> MNSPVDAPKWPRQIPYIIASE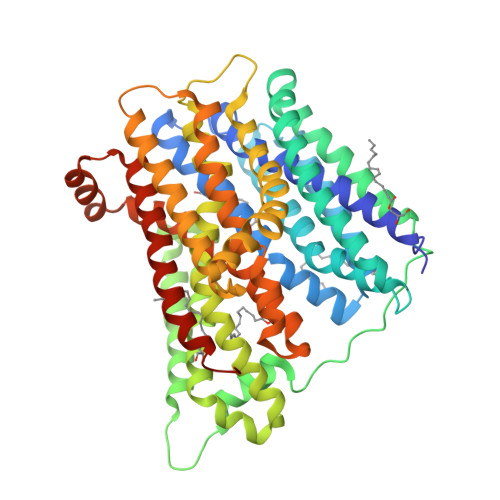ACERFSFYGMRNILTPFLMTALLLSIPEELRGAVAKDVFHSFVIGVYFFPLLGGWIADRFFGKYNTILWLSLIYCVGHAFLAIFEHSVQGFYTGLFLIALGSGGIKPLVSSFMGDQFDQSNKSLAQKAFDMFYFTINFGSFFASLSMPLLLKNFGAAVAFGIPGVLMFVATVFFWLGRKRYIHMPPEPKDPHGFLPVIRSALLTKVEGKGNIGLVLALIGGVSAAYALVNIPTLGIVAGLCCAMVLVMGFVGAGASLQLERARKSHPDAAVDGVRSVLRILVLFALVTPFWSLFDQKASTWILQANDMVKPQWFEPAMMQALNPLLVMLLIPFNNFVLYPAIERMGVKLTALRKMGAGIAITGLSWIVVGTIQLMMDGGSALSIFWQILPYALLTFGEVLVSATGLEFAYSQAPKAMKGTIMSFWTLSVTVGNLWVLLANVSVKSPTVTEQIVQTGMSVTAFQMFFFAGFAILAAIVFALYARSYQMQDHYRQATGSENLYFQ DNA polymerase μ incorporates nucleotides in the non-homologous end-joining (NHEJ) pathway of double-strand break (DSB) repair. Error-prone synthesis by pol μ often introduces mismatches, as well as short deletions or insertions, at repaired sites. Pol μ is expected to frequently encounter oxidized nucleotides in its biological roles. We employed time-lapse X-ray crystallography to obtain snapshots of 8-oxodGTP insertion by pol μ on a model DSB substrate.

We grew crystals of pol μ in complex with a model DSB substrate containing a single nucleotide gap with a templating C (Ct). We soaked pol μ-DNA binary complex crystals in a cryo solution containing 1 mM dGTP in the presence of catalytically inert Ca2+ (10 mM) to obtain pol μ-DNA-dGTP ternary complex crystals. We then solved the structure of the Ca2+-bound pre-catalytic ground state (GS) ternary complex of dGTP opposite template C (dGTP:Ct). The guanine base of dGTP(anti) forms Watson–Crick hydrogen bonds with Ct in anti-conformation. The methylene backbone of Lys438 stabilizes the guanine base. Arg445 forms hydrogen bonds with O2 of Ct(anti). The nucleotide (Can) and catalytic metal (Cac) sites are occupied by Ca2+. Metal coordination occurs through conserved active site aspartates 330, 332, and 418. The triphosphate of dGTP interacts with Gly320, Arg323, Lys325, and His329.Fig. 2 dGTP insertion opposite adenine and cytosine.

> GSAAAPLSPAWMPAYACQRPTPLTHHNTGLSEALEILAEAAGFEGSEGRLLTFCRAASVLKALPSPVTTLSQLQGLPHFGEHSSRVVQELLEHGVCEEVERVRRSERYQTMKLFTQIFGVGVKTADRWYREGLRTLDDLREQPQKLTQQQKAGLQHHQDLSTPVLRSDVDALQQVVEEAVGQALPGATVTLTGGFRRGKLQGHDVDFLITHPKEGQEAGLLPRVMCRLQDQGLILYHQHQHSCCESPTRLAQQSHMDAFERSFCIFRLPQPGSWKAVRVDLVVAPVSQFPFALLGWTGSKLFQRELRRFSRKEKGLWLNSHGLFDPEQKTFFQAASEEDIFRHLGLEYLPPEQRNA> MRSGSHHHHHHRSDITSLYKKAGLENLYFQGREDALRGFDALMATAGVESTIVKHAASGADSQTLNDELTRSLQLAHDRWGLGLLHL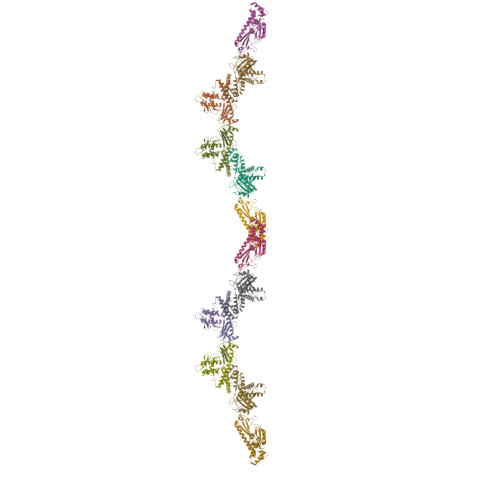RHEARLDRGEDTDVILLVDGREVARLSQGAAAISATYETMRAQNADDLSDWGVLPEGHRVTLKAGNNQMRVLVEDARDFETHWSSERGGAFVRTWRQGETLAVEVHRPASPGTALAKAAWKAIMSIKDRNFQRELMERSNSVGMLGALLGARHKDAGRALERLPEAHFAVRSTVVRMTGGAQREFDQWRSMVREGLDQLDELQKTTTRHLTEILRHGLK> GAMVYVFSTEM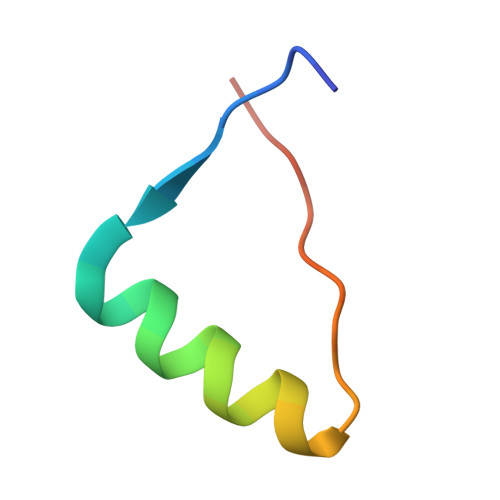ANKAAEAVLKGQVETIVSFHI> MSALPEEVNRTLLQIVQAFASPDNQIRSVAEKALSEEWITENNIEYLLTFLAEQAAFSQDTTVAALSAVLFRKLALKAPITHIRKEVLAQIRSSLLKGFLSERADSIRHKLSDAIAECVQDDLPAWPELLQALIESLKSGNPNFRESSFRILTTVPYLITAVDINSILPIFQSGFTDASDNVKIAAVTAFVGYFKQLPKSEWSKLGILLPSLLNSLPRFLDDGKDDALASVFESLIELVELAPKLFKDMFDQIIQFTDMVIKNKDLEPPARTTALELLTVFSENAPQMCKSNQNYGQTLVMVTLIMMTEVSIDDDDAAEWIESDDTDDEEEVTYDHARQALDRVALKLGGEYLAAPLFQYLQQMITSTEWRERFAAMMALSSAAEGCADVLIGEIPKILDMVIPLINDPHPRVQYGCCNVLGQISTDFSPFIQRTAHDRILPALISKLTSECTSRVQTHAAAALVNFSEFASKDILEPYLDSLLTNLLVLLQSNKLYVQEQALTTIAFIAEAAKNKFIKYYDTLMPLLLNVLKVNNKDNSVLKGKCMECATLIGFAVGKEKFHEHSQELISILVALQNSDIDEDDALRSYLEQSWSRICRILGDDFVPLLPIVIPPLLITAKATQDVGLIEEEEAANFQQYPDWDVVQVQGKHIAIHTSVLDDKVSAMELLQSYATLLRGQFAVYVKEVMEEIALPSLDFYLHDGVRAAGA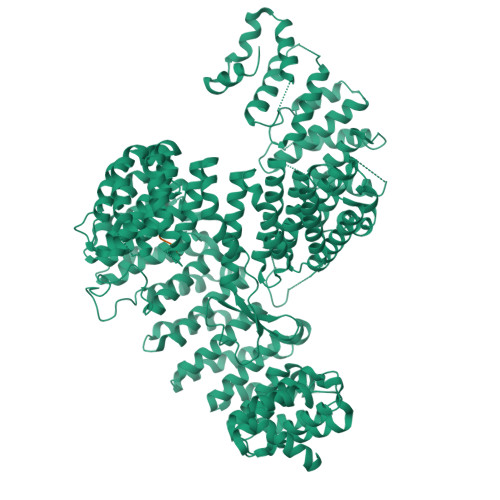TLIPILLSCLLAATGTQNEELVLLWHKASSKLIGGLMSEPMPEITQVYHNSLVNGIKVMGDNCLSEDQLAAFTKGVSANLTDTYERMQDRHGDGDEYNENIDEEEDFTDEDLLDEINKSIAAVLKTTNGHYLKNLENIWPMINTFLLDNEPILVIFALVVIGDLIQYGGEQTASMKNAFIPKVTECLISPDARIRQAASYIIGVCAQYAPSTYADVCIPTLDTLVQIVDFPGSKLEENRSSTENASAAIAKILYAYNSNIPNVDTYTANWFKTLPTITDKEAASFNYQFLSQLIENNSPIVCAQSNISAVVDSVIQALNERSLTEREGQTVISSVKKLLGFLPSSDAMAIFNRYPADIMEKVHKWFA;> TILRQLLPKNRRVTSGRRTTSAAGGIRKISGSIKK> MDSKDFLARLSLPARLASEQSGVPHHLILAQAALESGWGQRQILRENGEPSYNVFGVKATASWKGPVTEITTTEYENGEAKKVKAKFRVYSSYLEALS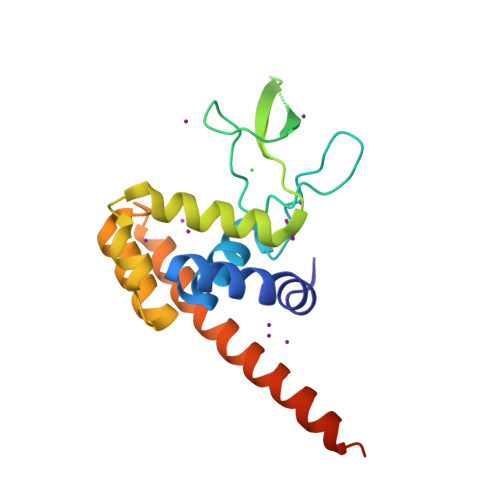DYVALLTRNPRYAAVTTAATAEQGAVALQNAGYATDPNYARKLTSMIQQLKAMSEKVSKTYSANLDNLFGSHHHHHH>[2x]MAQLALQMSSLGVEGEGIWLALGTIGMLLGMLYFIADGLDVQDPRQKEFYVITILIPAIAAASYLSMFFGFGLTEVSLANGRVV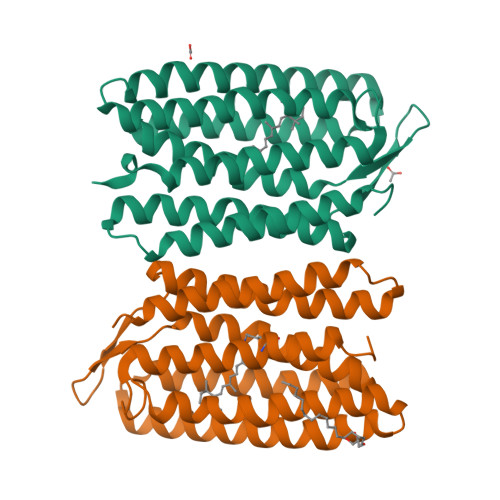DVYWARYADWLFTTPLLLLDIGLLAGASQRDIGALVGIDAFMIVTGLVATLTKVVVARYAFWTISTISMVFLLYYLVAVFGEAVSDADEDTRSTFNALRNIILVTWAIYPVAWLVGTEGLALTGLYGETLLFMVLDLVAKVGFGFILLRSRAIMGGGSEPTPSAQETAADLEHHHHHH> MRGSFANDATFEIKKCDLHRLEEGPPVTTVLTREDGLKYYRMMQTVRRMELKADQLYKQKIIRGFCHLCDGQEACCVGLEAGINPTDHLITAYRAHGFTFTRGLSVREILAELTGRKGGCAKGKGGSMHMYAKNFYGGNGIMGAQVPLGAGIALACKYNGKDEVCLTLYGDGAANQGQIFEAYNMAALWKLPCIFICENNRYGMGTSVERAAASTDYYKRGDFIPGLRVDGMDILCVREATRFAAAYCRSGKGPILMELQTYRYHGHSMSDPGVSYRTRE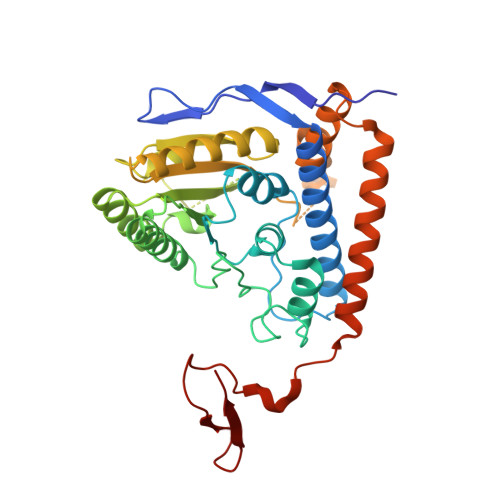EIQEVRSKSDPIMLLKDRMVNSNLASVEELKEIDVEVRKEIEDAAQFATADPEPPLEELGYHIYSSDPPFEVRGANQWIKFKSVS>ASLYEKLGGAAAVDLAVEKFYGKVLADERVNRFFVNTDMAKQKQHQKDFMTYAFGGTDRFPGRSMRAAHQDLVENAGLTDVHFDA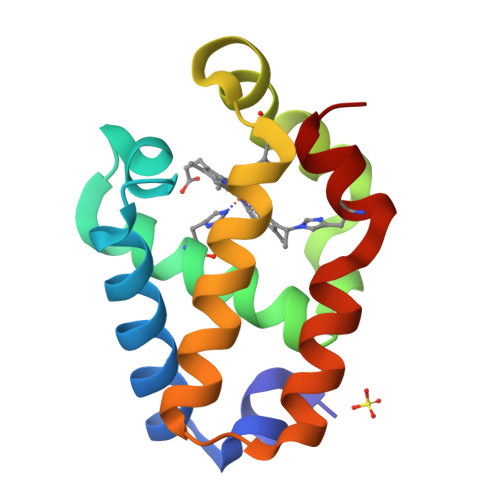IAENLVLTLQELNVSQDLIDEVVTIVGSVQHRNDVLNR[3x]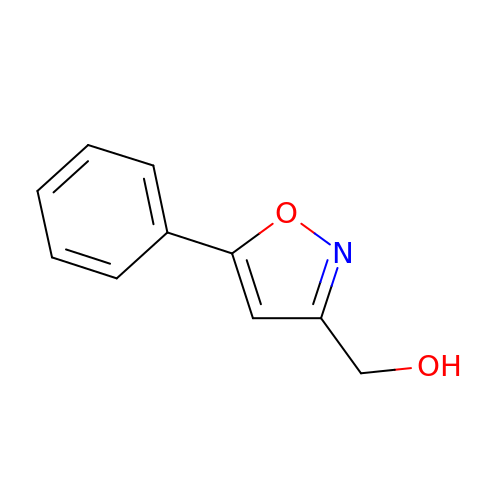(5-phenyl-1,2-oxazol-3-yl)methanol | C10 H9 N O2 | BPAFLGGUEBMWRN-UHFFFAOYSA-N> MQCMAFHQFAPSSSLPIWSSINNRFTPKTSITSISKPKPKLKPKSNLKSRSRSSTCYPIQCTVVDNPSSTITNNSDRRSANYGPPIWSFDFIQSLSTQYKGELYTSRLNKLEKDVKRILVGEENCLAQLELIDTIQRLGLSYRFENEIISILKEKFTNNNNNPNYDLYATALQFRLLRQYGFEVPQEIFNNFKDQKTGEFKANISNDIMGALGLYEASFYGKKGESILDEARIFTTKCLKNYIEKNKLLDDDNNIIALFVNHALETPLHWRIN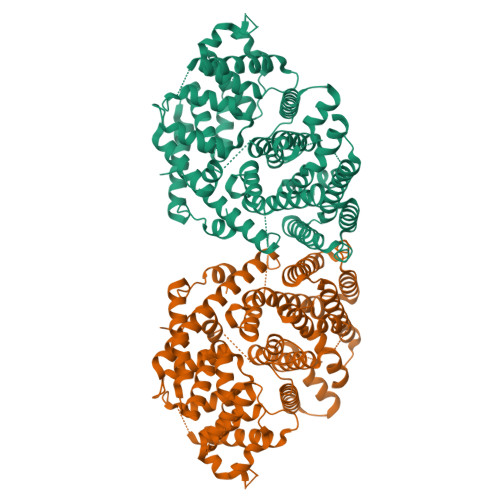RLEARWFIEMYQKKKDMNFTLLEFAKLDFNMLQSIHQEDLKHLSRWWEQSKLGEKKMENYVRDRLVEAFLWQIGVKFEPQFSQFRRISARLYVLITVIDDIYDVYGTLEELELFTKAIERWDVKAINELPEYMRMPFFFLFNTVNEMGYDTLTDKNFINIEYLKKSWVVWSKYQLEEAKWFYSGYKPTLEEYMKNTWISVGGPIILLHAYFAFTNPLEKASIKFLEEGYDDPSINIHEGSLEISNDGYPTIFHLGSILLRLEDDLGTSSDEMKRGDVPKSIQCYMSDTGVSEDEAREHIKFLIMETWKEMNKEMDFNNYFSKEVVHVCKNLGRTAKFIYLYGDGHASQNNLSKGHISDLIINPIPM> MKIKRFGRIREVIPLPPLTEIQVESYKKALQADVPPEKRENVGIQAAFKETFPIEEGDKGKGGLVLDFLEYRIGDPPFSQDECREKDLTYQAPLYARLQLIHKDTGLIKEDEVFLGHLPLMTEDGSFIINGADRVIVSQIHRSPGVYFTPDPARPGRYIASIIPLPKRGPWIDLEVEASGVVTMKVNKRKFPLVLLLRVLGYDQETLVRELSAYGDLVQGLLDEAVLAMRPEEAMVRLFTLLRPGDPPKKDKALAYLFGLLADPKRYDLGEAGRYKAEEKLGVGLSGRTLVRFEDGEFKDEVFLPTLRYLFALTAGVPGHEVDDIDHLGNRRIRTVGELMADQFRVGLARLARGVRERMVMGSPDTLTPAKLVNSRPLEAALREFFSRSQLSQFKDETNPLSSLRHKRRISALGPGGLTRERAGFDVRDVHRTHYGRICPVETPEGANIGLITSLAAYARVDALGFIRTPYRRVKNGVVTEEVVYMTASEEDRYTIAQANTPLEGDRIATDR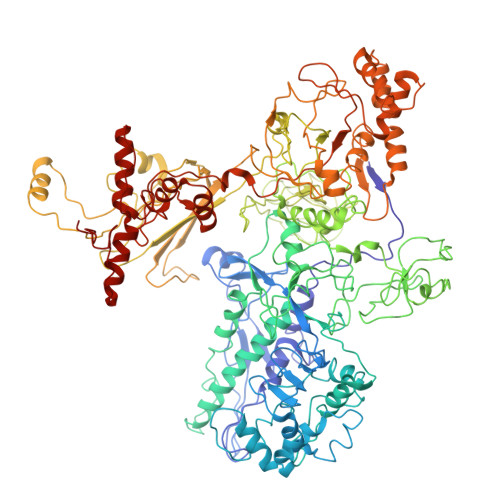VVARRRGEPVIVAPEEVEFMDVSPKQVFSLNTNLIPFLEHDDANRALMGSNMQTQAVPLIRAQAPVVMTGLEERVVRDSLAALYAEEDGEVVKVDGTRIAVRYEDGRLVEHPLRRYARSNQGTAFDQRPRVRVGQRVKKGDLLADGPASEEGFLALGQNVLVAIMPFDGYNFEDAIVISEELLKRDFYTSIHIERYEIEARDTKLGPERITRDIPHLSEAALRDLDEEGIVRIGAEVKPGDILVGRTSFKGEQEPSPEERLLRSIFGEKARDVKDTSLRVPPGEGGIVVGRLRLRRGDPGVELKPGVREVVRVFVAQKRKLQVGDKLANRHGNKGVVAKILPVEDMPHLPDGTPVDVILNPLGVPSRMNLGQILETHLGLAGYFLGQRYISPVFDGATEPEIKELLAEAFNLYFGKRQGEGFGVDKREKEVLARAEKLGLVSPGKSPEEQLKELFDLGKVVLYDGRTGEPFEGPIVVGQMFIMKLYHMVEDKMHARSTGPYSLITQQPLGGKAQFGGQRFGEMEVWALEAYGAAHTLQEMLTIKSDDIEGRNAAYQAIIKGEDVPEPSVPESFRVLVKELQALALDVQTLDEKDNPVDIFEGLASKR> QINQV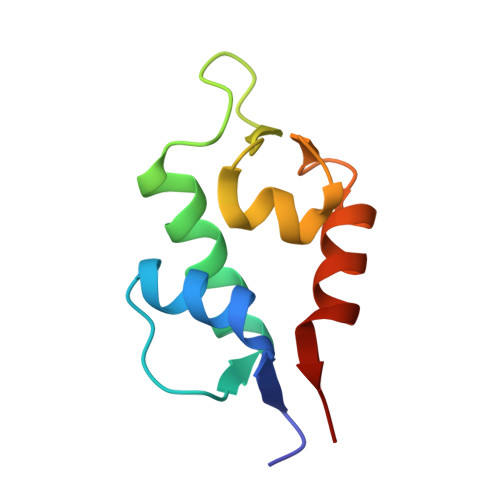RPKLPLLKILHAAGAQGEMFTVKEVMHYLGQYIMVKQLYDQQEQHMVYCGGDLLGELLGRQSFSVKDPSPLYDMLRKNLVTLAT> GAMDYTLRKIKIAAAHSLSLGLLPTIVKQMPTQFTYAVEAIDVDQAVDMLREGQSDFIFSYHDENLQQAPFDNIRLFESRLFPVCANNGRGEPRYTLEQPHFPLLNYSQNSYMGRLINRTLTRHAELSFSTFFVSSMSELLKQVAMDGCGIAWL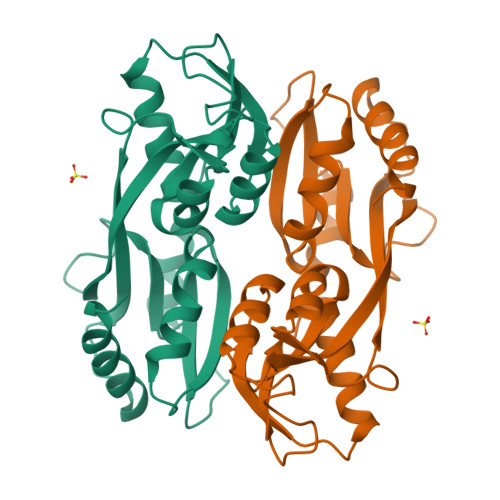PEYAIRQEITDGRLIVLDADELVIPIQAYAYRMNTRMSQVAETFWRDLRGLQAAL OCTANOIC ACID (2-HYDROXY-1-HYDROXYMETHYL-HEPTADEC-3-ENYL)-AMIDE 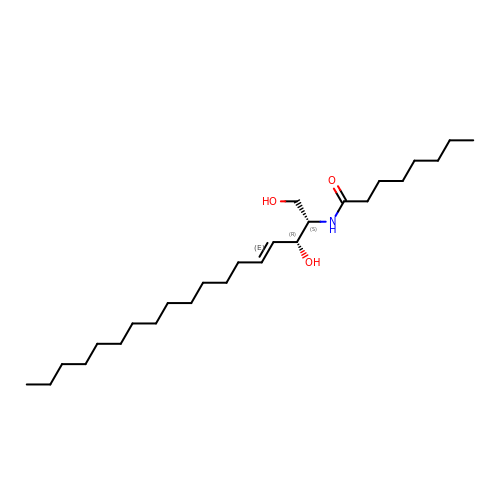| C26 H51 N O3 | APDLCSPGWPLYEQ-WUBHUQEYSA-N> GAMEEERHQVLKKWNETAHPHPEENFLQLFEKQAERIPEAIAVICEDQALSYTELNQQANRLAHFLMEYGVGPEQYVALALPRSAEMVIAMLAVLKTGAAYLPLDLDYPDERIAFMLEDTKPVCIVTSSSVQSKLSHFPSCSTIILDHPETEQAIKHYPDTNVPKTQSPLHPAYVIYTSGSTGKPKGVVVPFHSLNNFLLAMREKFALKEHDRLLAVTTIAFDISALEIFLPLISGASLVVAKKETIQDPQALAAVISDKEITIMQATPTLWHMLVTHHPDCIAGLRVLVGGEALSSGLASALHRLACEVTNLYGPTETTIWSTMSPLHPDDARAPSIGRPIWNTQVYVLDEQLQPVPPGVVGELYIAGSGLARGYLRRPDLTAERFVANPYGPPGSRMYRTGDLVRWRMDGSLDYIGRVDHQIKLRGFRIEIGEIEAVLSQCDLVERALVVAREDQPGDQRLVAYVIPCEQSKGTLDLAELRRYVSERLPDYMVPSAFMVLNEFPLTPNGKIDRKALPAPDFTMTVKGRKPRNPQEEILCELFAEVLEIPVVGIDDHFFELGGHSLLAARLISRIRDVLGVEITIGKLFASPTVASLVKHLEDAENRKPPVKAYACKEDIPLSFAQRRLWFLYHLEGPSPTYNIPVVVHLTGELHYQALQQA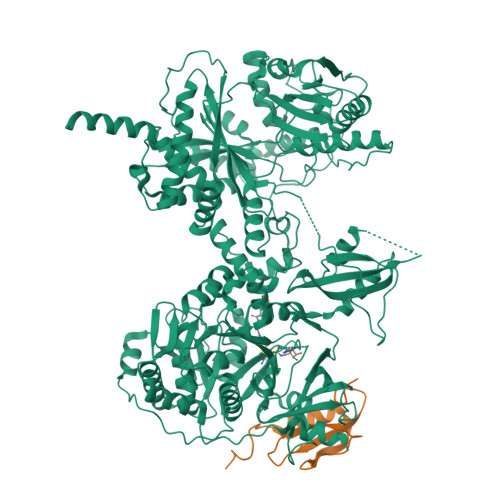LYDVIERHEPLRTIFPEHSGASRQVILEPHQARPELMIKEISESELSDELNAAVRYRFDLAAEPAIRAQLFVLGPNRHVLLLLMHHMIVDGWSLTPLTRDIAAAYNAHCRNQKVEWAPLPVKYADYALWQQEILGDETNPDSLIAKQLDYWKKTLAGLPEELELPTDYPRPAESSYEGGIVDFCMDAELHKRLLDLARENKASLFMVLQAGFAAFLTRLGAGTDIPIGSPIAGRNDDSLEHLVGLFINTLVLRMDTSGNPSFRELLGRVREVNLSAYENQDIPFERLVEILNPVRSRAKHPLFQVMFVFQNTPEPKLELQGLESRLEIRSVGTAKFDLTLELRERRGEDGSPDGLIGLFEYSRDLFDHTTVEAFAKRLCQLLREVVMNPDLPIGQIDMLLPEERKKLLAAAENLYFQ;> GAMGMTNPFENKEGTYLVLINDEGQYSLWPASIAIPPGWNIAFAENTRSACLDYINAHWIDMRPNSLKDGSLSKRDNDYSGVK> MNSSKETKSEPSDSKKLMDQPYSKTDFLMGTVVTLKIYDKGKEDVLDKGFDRIKDLAAKITTSDSEKTSEVDKINEQAGKKPVKVSEDVYYLIQEGLKYSENSGGSFDITIGPLTSLWHIGFSDARKPSQAEIDAVLPLINYKDVKMNDKDQTVYLEKEGMELDLGAIAKGFITDETLKVFKENKVTTSIIDLGGNIYVQGNNPNGNKWNVGIQDPFSPRGSVIGKLPESNMSIVTSGIYERYLEVDGKTYHHILDPKTGYPFDNDIAGVSIVSKKSIDGDGLSTATFSKGIKGGMDYIEQFEGVDAIFISKEKKVYETSGLKGQFELTDKDFQMDTLKK

A Mg2+‐dependent protein flavin mononucleotide (FMN) transferase (FmnB; UniProt: LMRG_02181) in EET is responsible for the transfer of electrons from intracellular to extracellular by hydrolyzing cofactor flavin adenine dinucleotide (FAD) and transferring FMN. FmnB is a flavin transferase belonging to ApbE family; it hydrolyzes flavin adenine dinucleotide (FAD) and converts flavin mononucleotide (FMN) to pheromone lipoprotein (PplA; UniProt: LMRG_02182), and divalent cations are required this process. Here, we report a series of crystal structures of apo‐FmnB and FmnB complexed with substrate FAD, three inhibitors AMP, ADP, and ATP, revealing the unusual catalytic triad center (Asp301‐Ser257‐His273) of FmnB. Notably, the structures of FmnB in complex with distinct inhibitors, together with biochemical assays, revealed that all three inhibitors indeed inhibited the activity of FmnB by occupying the binding site of the FAD substrate.

As defined by unbiased electron density, FAD in a bent conformation binds to the central cavity of FmnB with the diphosphate nearly perpendicular to the adenine. The adenine of FAD is buried deep in the hydrophobic pocket inside the cavity, and the isoalloxazine ring is exposed outside the hydrophobic cavity. The adenine of FAD forms hydrogen bonds with Ser126 and Leu275 of FmnB and establishes water‐mediated hydrogen bonds with the carbonyl group on the main chain of Asp184. Additionally, the sugar ring of FAD forms salt bridges with His273 and Arg262 and hydrogen bonds with the side chain of Asp184. Instead, the isoalloxazine ring is sandwiched between Phe142 and Met49 through the hydrophobic interactions. Remarkably, Arg262 not only forms a salt bridge with the sugar ring but also forms water‐mediated hydrogen bonds with isoalloxazine ring, which likely maintains the curved conformation of FmnB‐bound FAD. Moreover, the diphosphate of FAD is inserted further into the FAD‐binding pocket, forming hydrogen bonds with Ser257 and water‐mediated hydrogen bonds with His273 and coordinating with Mg2+ through Asp301. Two Mg2+ ions are present in the electron density model, and they are coordinated with the phosphate groups as well as water molecules. In addition to these interactions, one of the Mg2+ ions (Mg1) coordinates with Asp301, Ser304, and Ala187. Glu261 adopted a rotamer conformation that removed it from the catalytic center through charge repulsion, and Arg262 no longer occupied the position of the sugar ring but formed a salt bridge with the sugar ring to stabilize the FAD conformation.> MDKDCEMKRTTLDSPLGKLELSGCEQGLHEIKLLGKGTSAADAVEVPAPAAVLGGPEPLMQCTAWLNAYFHQPEAIEEFPVPALHHPVFQQESFTRQVLWKLLKVVKFGEVISYQQLAALAGNPKAARAVGGAMRGNPVPILIPCHRVVCSSGAVGNYSGGLA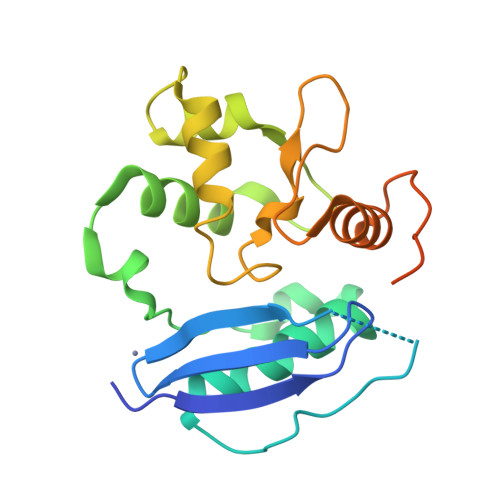VKEWLLAHEGHRLGKPGLGGSSGLAGAWLKGAGATSGSPPAGRN> GPGYQMADEIDAMALYRAWQQLDNGSCAQIRRVSEPDELRDIPAFYRLVQPFGWENPRHQQALLRMVFCLSAGKNVIRHQDKKSEQTTGISLGRALANSGRINERRIFQLIRADRTADMVQLRRLLTHA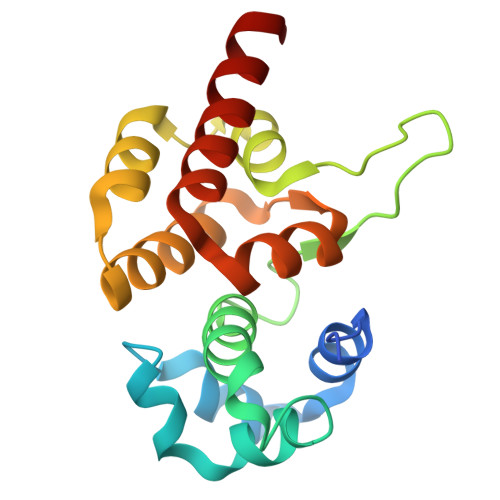EPVLDWPLMARMLTWWGKRERQQLLEDFVLTTNKNA>MELHHHHHHEEMPFKPLVTAGIESLLNTFLYRSPALKTARSRLLGKVLRVEVKGFSTSLILVFSERQVDVLGEWAGDADCTVIAYASVLPKLRDRQQLTALIRSGELEVQGDIQVVQNFV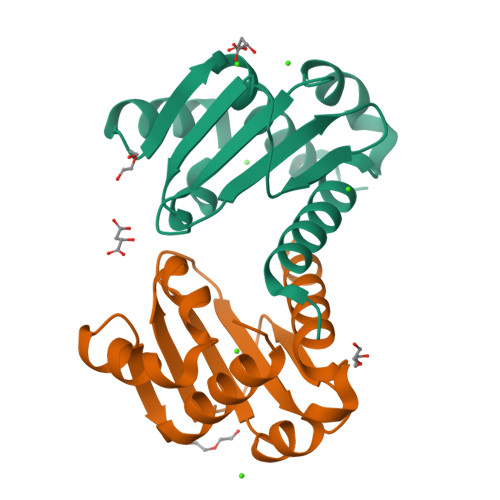ALADLAEFDPA[2x]>[2x]MGSDKIHHHHHHMTVRTRVTDLLEIEHPILMGGMAWAGTPTLAAAVSEAGGLGIIGSGAMKPDDLRKAISELRQKTDKPFGVNIILVSPWADDLVKVCIEEKVPVVTFGAGNPTKYIRELKENGTKVIPVVASDSLARMVERAGADAVIAEGMESGGHIGEVTTFVLVNKVSRSVNIPVIAAGGIADGRGMAAAFALGAEAVQMGTRFVASVESDVHPV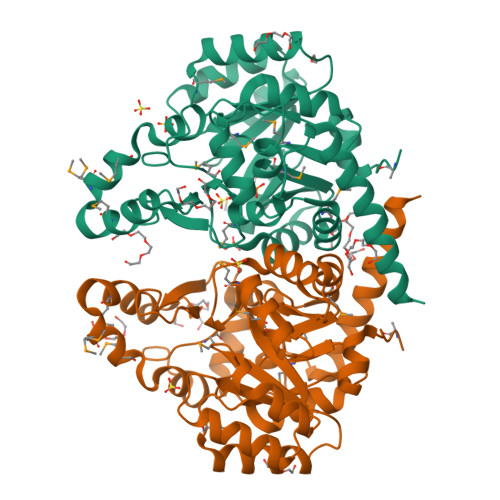YKEKIVKASIRDTVVTGAKLGHPARVLRTPFARKIQEMEFENPMQAEEMLVGSLRRAVVEGDLERGSFMVGQSAGLIDEIKPVKQIIEDILKEFKETVEKLRGYIEE> MRSIRGVCCFSSLYTTQFRVHATYDVAPLSHKELFSIYQNWDKTRDELDLLEEVEERISKWKLNKWEMRIPPLLTAREKELMRQQQELLKSIFFDWGKCRDALNKDLELISSITGLPKGTVREKNRAWLQEEAAKLRWVGEVSKATRLRDAFLRLEVYGSRDHRLLERLCCIYGLGLQGSFESAFSNYIVEDPITKKIYVDEKNSFRDLLAYIIHTYPQIDIIYDFLGFNFIGGYRSSLRRYLECMVSRSTEGEKI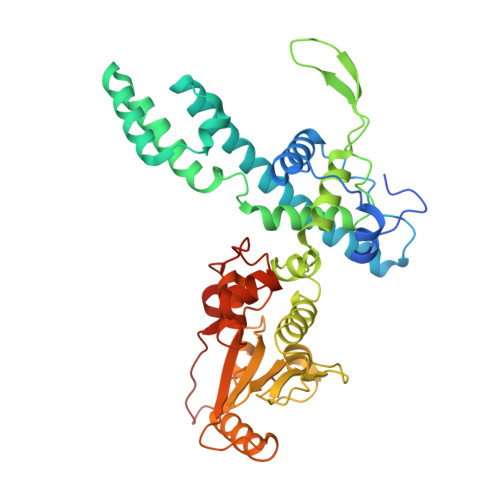PGRLVFGRGKPAEILFDFGNSNESLVSGECTQGFPDFVFVKGSDMTLIIIASENSWLRNRQLPHRKQMEGIARRASFVLGIPFSEVRVRNLLLPPTYLDKDSIVRINEAVLGLSKEEQRNLAPWLEMYQKELDSKDVDFCSLMKSTNEEEWLTL> TEEPDFTALCQKLKIPDHVRERAWLTWEKVSSVDGVLGGYIQKKKELWGICIFIAAVDLDEMSFTFTELQKNIEISVHKFFNLLKEIDTSTKVDNAMSRLLKKYDVLFALFSKLERTCELIYLTQ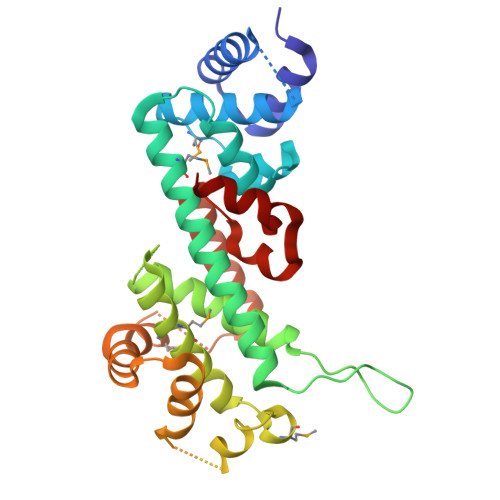PSSSISTEINSALVLKVSWITFLLAKGEVLQMEDDLVISFQLMLCVLDYFIKLSPPMLLKEPYKTAVIPINGSPRTPRRGQNRSARIAKQLENDTRIIEVLCKEHECNIDEVKNVYFKNFIPFMNSLGLVTSNGLPEVENLSKRYEEIYLKNKDLDARLFLDHDKTLQTDSIDSFETQR>MSKIESALQAAQPGLSRLRGGAGGMGYRAATTQAEQPRSSLLDTIGRFAKAGADMYTAKEQRARDLADERSNEIIRKLTPEQRREALNNGTLLYQDDPYAMEALRVKTGRNAAYLVDDDVMQKIKEGVFRTREEMEEYRHSRLQEGAKVYAEQFGIDPEDVDYQRGFNGDITERNISLYGAHDNFLSQQAQKGAIMNSRVELNGVLQDPDMLRRPDSADFFEKYIDNGLVTGAIPSDAQATQLISQAFSDASSRAGGADFLMRVGDKKVTLNGATTTYRELIGEEQWNALMVTAQRSQFETDAKLNEQYRLKINSALNQEDPRTAWEMLQGIKAELDKVQPDEQMTPQREWLISAQEQVQNQMNAWTKAQAKALDDSMKSMNKLDVIDKQFQKRINGEWVSTDFKDMPVNENTGEFKHSDMVNYANKKLAEIDSMDIPDGAKDAMKLKYLQADSKDGAFRTAIGTMVTDAGQEWSAAVINGKLPERTPAMDALRRIRNADPQLIAALYPDQAELFLTMDMMDKQGIDPQVILDADRLTVKRSKEQRFEDDKAFESALNASKAPEIARMPASLRESARKIYDSVKYRSGNESMAMEQMTKFLKESTYTFTGDDVDGDTVGVIPKNMMQVNSDPKSWEQGRDILEEARKGIIASNPWITNKQLTMYSQGDSIYLMDTTGQVRVRYDKELLSKVWSENQKKLEEKAREKALADVNKRAPIVAATKAREAAAKRVREKRKQTPKFIYGRKE[6x];>[6x]MDKYDKNVPSDYDGLFQKAADANGVSYDLLRKVAWTESRFVPTAKSKTGPLGMMQFTKATAKALGLRVTDGPDDDRLNPELAINAAAKQLAGLVGKFDGDELKAALAYNQGEGRLGNPQLEAYSKGDFASISEEGRNYMRNLLDVAKSPMAGQLETFGGITPKGKGIPAEVGLAGIGHKQKVTQELPESTSFDVKGIEQEATAKPFAKDFWETHGETLDEYNSRSTFFGFKNAAEAELSNSVAGMAFRAGRLDNGFDVFKDTITPTRWNSHIWTPEELEKIRTEVKNPAYINVVTGGSPENLDDLIKLANENFENDSRAAEAGLGAKLSAGIIGAGVDPLSYVPMVGVTGKGFKLINKALVVGAESAALNVASEGLRTSVAGGDADYAGAALGGFVFGAGMSAISDAVAAGLKRSKPEAEFDNEFIGPMMRLEARETARNANSADLSRMNTENMKFEGEHNGVPYEDLPTERGAVVLHDGSVLSASNPINPKTLKEFSEVDPEKAARGIKLAGFTEIGLKTLGSDDADIRRVAIDLVRSPTGMQSGASGKFGATASDIHERLHGTDQRTYNDLYKAMSDAMKDPEFSTGGAKMSREETRYTIYRRAALAIERPELQKALTPSERIVMDIIKRHFDTKRELMENPAIFGNTKAVSIFPESRHKGTYVPHVYDRHAKALMIQRYGAEGLQEGIARSWMNSYVSRPEVKARVDEMLKELHGVKEVTPEMVEKYAMDKAYGISHSDQFTNSSIIEENIEGLVGIENNSFLEARNLFDSDLSITMPDGQQFSVNDLRDFDMFRIMPAYDRRVNGDIAIMGST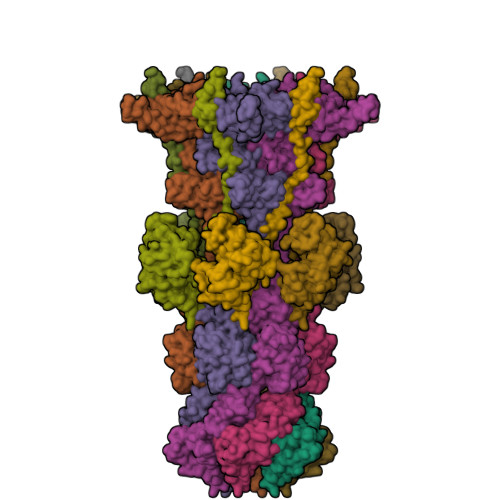GKTTKELKDEILALKAKAEGDGKKTGEVHALMDTVKILTGRARRNQDTVWETSLRAINDLGFFAKNAYMGAQNITEIAGMIVTGNVRALGHGIPILRDTLYKSKPVSAKELKELHASLFGKEVDQLIRPKRADIVQRLREATDTGPAVANIVGTLKYSTQELAARSPWTKLLNGTTNYLLDAARQGMLGDVISATLTGKTTRWEKEGFLRGASVTPEQMAGIKSLIKEHMVRGEDGKFTVKDKQAFSMDPRAMDLWRLADKVADEAMLRPHKVSLQDSHAFGALGKMVMQFKSFTIKSLNSKFLRTFYDGYKNNRAIDAALSIITSMGLAGGFYAMAAHVKAYALPKEKRKEYLERALDPTMIAHAALSRSSQLGAPLAMVDLVGGVLGFESSKMARSTILPKDTVKERDPNKPYTSREVMGAMGSNLLEQMPSAGFVANVGATLMNAAGVVNSPNKATEQDFMTGLMNSTKELVPNDPLTQQLVLKIYEANGVNLRERRK>MQPTAIRLEDYDKSKLRLPFESPYFPAYFRLLKWKFLDVCVESTRNNDIGYFKLFESLFPPGKLEEIARMIIDEPTPVSHDPDMIKIRNADLDVKIRKQAETYVTLRHAHQQKVQRRRFSECFLNTVLFDEKGLRIADEVMFNYDKELYGYSHWE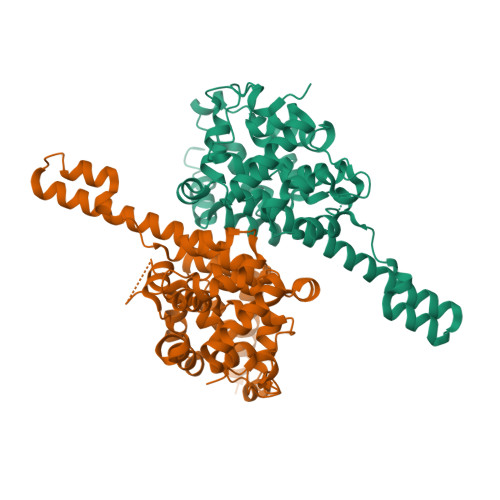DLPDGWLTAETFKNKFYDEEEVTNNPFGYQKLDRVAGAARGMIIMKHLKSNPRCVSETTILAFEVFNKGNHQLSTDLVEDLLTEGPAFELKIENGEEKKYAVKKWSLHKTLTMFLAIIGFKSNDKKEKNEHEEWYYGFIDAMKNDPANRAALYFLDKNWPEELEEREKERDRIRLTLLKS[2x]> GHMLRLSAPGQLDDDLCLLGDVQVPVFLLRLGEASWALVEGGISRDAELVWADLCRWVADPSQVHYWLITHKHYDHCGLLPYLCPRLPNVQVLASERTCQAWKSESAVRVVERLNRQLLRAEQRLPEACAWDALPVR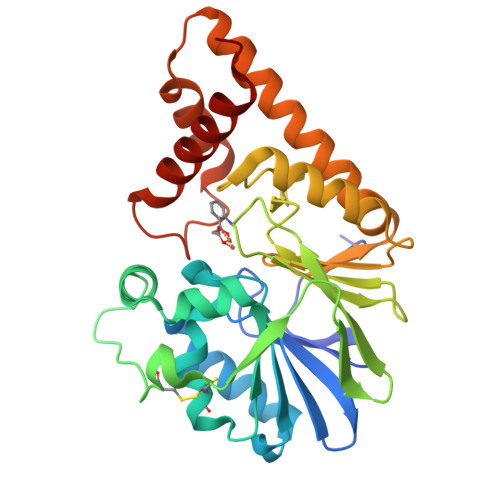AVADGEWLELGPRHRLQVIEAHGHSDDHVVFYDVRRRRLFCGDALGEFDEAEGVWRPLVFDDMEAYLESLERLQRLPTLLQLIPGHGGLLRGRLAADGAESAYTECLRLCRRLLWRQSMGESLDELSEELHRAWGGQSVDFLPGELHLGSMRRMLEILSRQALPLD> MELLLLSNSTLPGKAWLEHALPLIANQLNGRRSAVFI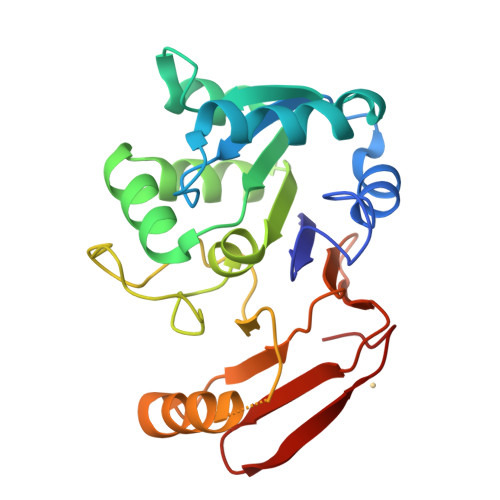PFAGVTQTWDEYTDKTAEVLAPLGVNVTGIHRVADPLAAIEKAEIIIVGGGNTFQLLKESRERGLLAPMADRVKRGALYIGWSAGANLACPTIRTTNDMPIVDPNGFDALDLFPLQINPHFTNALPEGHKGETREQRIRELLVVAPELTVIGLPEGNWIQVSNGQAVLGGPNTTWVFKAGEEAVALEAGHRF(2R)-butane-1,2,4-tricarboxylic acid | C7 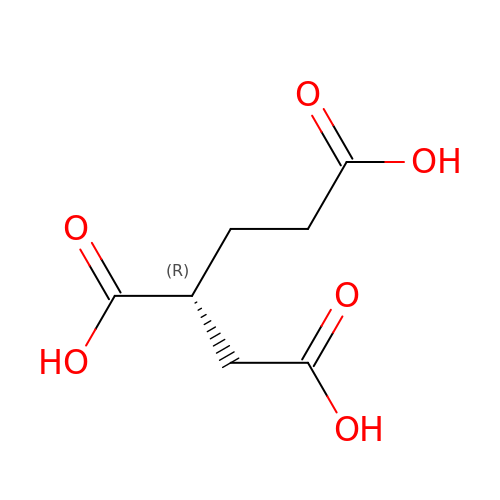H10 O6 | LOGBRYZYTBQBTB-SCSAIBSYSA-N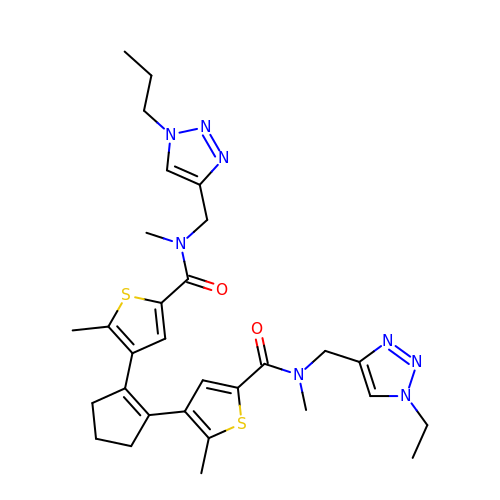~{N}-[(1-ethyl-1,2,3-triazol-4-yl)methyl]-~{N},5-dimethyl-4-[2-[2-methyl-5-[methyl-[(1-propyl-1,2,3-triazol-4-yl)methyl]carbamoyl]thiophen-3-yl]cyclopenten-1-yl]thiophene-2-carboxamide | C30 H38 N8 O2 S2 | GGDTYYUIMGUGDO-UHFFFAOYSA-N> MSMNYAAGLSPYADKGKCGLPEIFDPPEELERKVWELARLVWQSSSVVFHTGAGISTASGIPDFRGPHGVWTMEERGLAPKFDTTFESARPTQTHMALVQLERVGLLRFLVSQNVDGLHVRSGFPRDKLAELHGNMFVEECAKCKTQYVRDTVVGTMGLKATGRLCTVAKARGLRACRGELRDTILDWEDS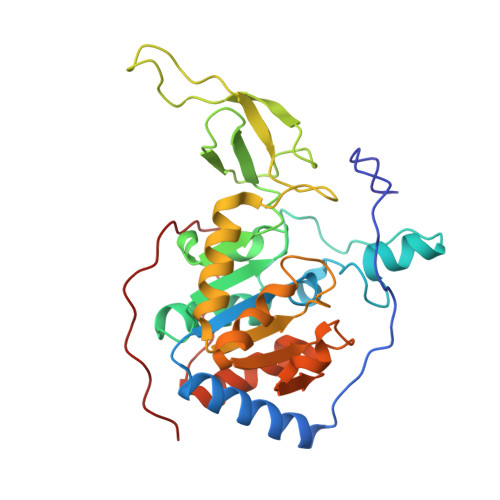LPDRDLALADEASRNADLSITLGTSLQIRPSGNLPLATKRRGGRLVIVNLQPTKHDRHADLRIHGYVDEVMTRLMKHLGLEIPAWDGPRVLERALPPLPRPPTPK> MGHHHHHHSAKQTGYLTIGGQRYQ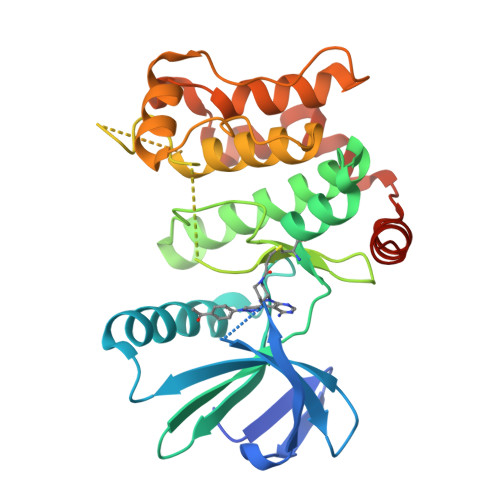AEINDLENLGEMGSGTCGQVWKMRFRKTGHVIAVKQMRRSGNKEENKRILMDLDVVLKSHDCPYIVQCFGTFITNTDVFIAMELMGTCAEKLKKRMQGPIPERILGKMTVAIVKALYYLKEKHGVIHRDVKPSNILLDERGQIKLCDFGISGRLVDSKAKTRSAGCAAYMAPERIDPPDPTKPDYDIRADVWSLGISLVELATGQFPYKKCKTDFEVLTKVLQEEPPLLPGHMGFSGDFQSFVKDCLTKDHRKRPKYNKLLEHSFIKRYETLEVDVASWFKDVMAKTESPRTSG> KVVKFSYMWTINNFSFCREEMGEVIKSSTFSSGANDKLKWCLRVNPKGLDEESKDYLSLYLLLVSCPKSEVRAKFKFSILNAKGEE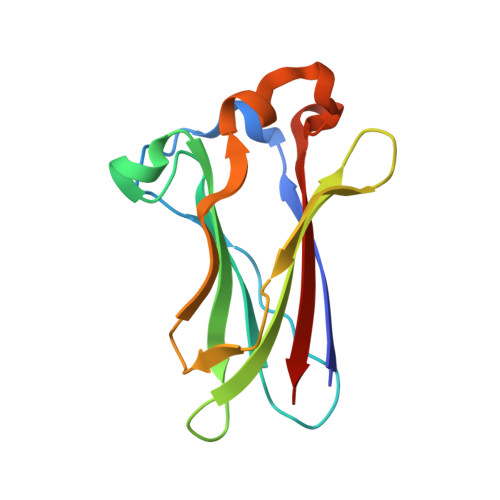TKAMESQRAYRFVQGKDWGFKKFIRRDFLLDEANGLLPDDKLTLFCEVSVVQD> SLGSLTIAEPAMIAECKTRTEVFEISRRLIDRTNANFLVWPPCVEV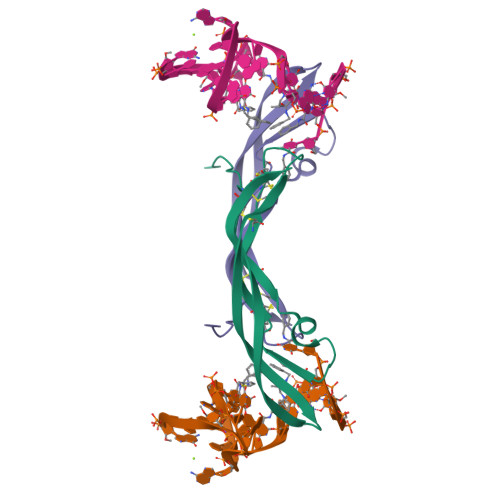QRCSGCCNNRNVQCRPTQVQLRPVQVRKIEIVRKKPIFKKATVTLEDHLACKCETV> GTTEGDEEDATEAWRLHQKHVFVLSEAGKPVYSRYGSEEALSSTMGVMVALVSFLEADKNAIRSIHADGYKVVFVRRSPLVLVAVARTRQSAQELAQELLYIYYQILSLLTGAQLSHIFQQKQNYDLRRLLSGSERITDNLLQLMARDPSFLMGAARCLPLAAAVRDTVSASLQQARARSLVFSILLARNQLVALVRRKDQFLHPIDLHLLFNLISSSSSFREGEAWTPVCLPKFNAAGFFHAHISYLEPDTDLCLLLVSTDREDFFAVSDCRRRFQERLRKRGAHLALREALRTPYYSVAQVGIPDLRHFLYKSKSSGLFTSPEIEAPYTSEEEQERLLGLYQYLHSRAHNASRPLKT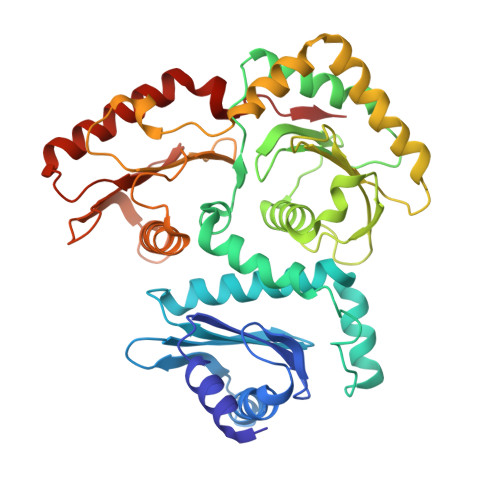IYYTGPNENLLAWVTGAFELYMCYSPLGTKASAVSAIHKLMRWIRKEEDRLFILTPLTY> 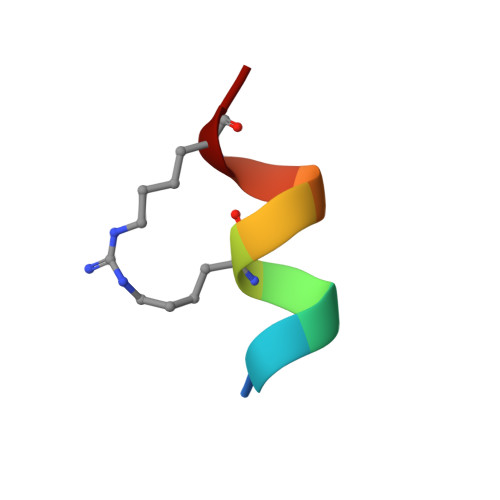HKILLRLLRX> SNIPLEELQRNLQFHAFISYSGHDSFWVKNELLPNLEKEGMQICLHERNFVPGKSIVENIITCIEKSYKSIFVLSPNFVQSEWCHYELYFAHHNLFHEGSNSLILILL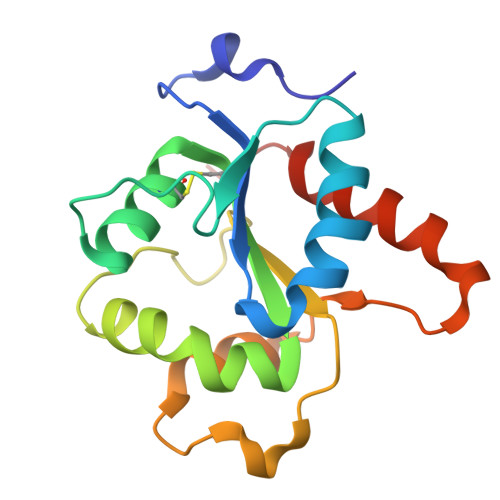EPIPQYSIPSSYHKLKSLMARRTYLEWPKEKSKRGLFWANLRAAINIKLTEQAK The chitinase Chit42 from T. harzianum (orthologous to Ech42) plays an important role in the fungus anti-phytopathogens activity. Chitinase Chit42 from Trichoderma harzianum hydrolyses chitin oligomers with a minimal of three N-acetyl-d-glucosamine (GlcNAc) units. Chitinases from GH18 are retaining enzymes, which means that the β-anomeric configuration found in the substrate is retained in the product, showing an unusual substrate-assisted catalytic mechanism where the acid protonating the glycosidic bond (to be hydrolysed) is a conserved glutamate residue (included in the DXXDXDE sequence), and the nucleophile is the oxygen of the N-acetyl group (of GlcNAc) on the subsite − 1 sugar. All chitinases described in yeast and fungi are included in the family GH18.

We have modeled a chitooligosaccharide within the active site channel by structural superimposition of the reported complex of this substrate with the Serratia marcescens ChiA-D313A mutant onto the coordinates of Chit42 here presented. Although ChiA and Chit42 sequences are only 26% similar, the corresponding residues located at the active site are rather conserved. Therefore, the distorted conformation of the substrate at the cleavage point observed for ChiA fits well within the Chit42 active site groove. First of all, the substrate is tightly recognized at subsites − 4 to + 2 by a net of hydrogen links to several Chit42 residues. Therefore, there are at least 6 substrate-binding subsites in this protein. According to our complex model, Glu316 is hydrogen linked to O3 of the sugar at subsite − 2, but seems also able to link to a free amine group by a slight switch of its side-chain, therefore compensating the loss of the hydrogen bond to Trp378 and contributing to stabilized a deacetylated sugar at this subsite − 2. According to our model, Arg52 is also involved in allocating the sugar at this subsite; therefore, its flexible chain provides additional plasticity to the sugar type occupying this binding subsite. A last interesting feature is the fact that the side-chain of Trp131, making subsite + 1, presents rather weak electron density in our solved free enzyme crystal, revealing a marked disorder.

> MLSFLGKSVALLAALQATLSSPKPGHRRASVEKRANGYANSVYFTNWGIYDRNFQPADLVASDVTHVIYSFMNLQADGTVISGDTYADYEKHYADDSWNDVGTNAYGCVKQLFKVKKANRGLKVLLSIGGWTWSTNFPSAASTDANRKNFAKTAITFMKDWGFDGIDIDWEYPADATQASNMILLLKEVRSQLDAYAAQYAPGYHFLLTIAAPAGKDNYSKLRLADLGQVLDYINLMAYDYAGSFSPLTGHDANLFNNPSNPNATPFNTDSAVKDYINGGVPANKIVLGMPIYGRSFQNTAGIGQTYNGVGSGSWEAGIWDYKALPKAGATVQYDSVAKGYYSYNSATKELISFDTPDMINTKVAYLKSLGLGGSMFWEASADKKGADSLIGTSHRALGGLDTTQNLLSYPNSKYDNIKNGLN>[2x]MLANENSLLTMFRELGSGKLPLQIEQFERGKTIFFPGDPAERVYLLVKGAVKLSRVYESGEEITVALLRENSVFGVLSLLTGQRSDRFYHAVAFT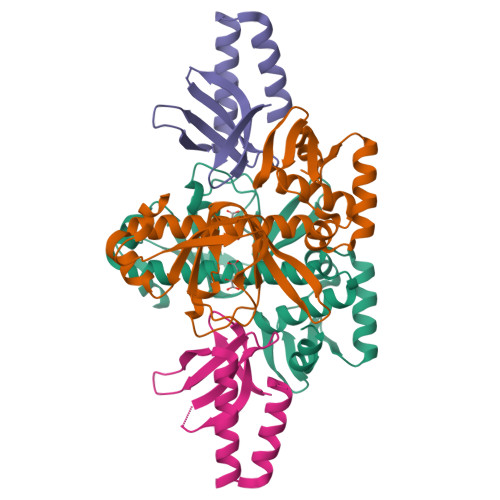PVQLFSVPIEFMQKALIERPELANVMLQGLSSRILQTEMMIETLAHRDMGSRLVSFLLILCRDFGIPSPDGITIDLKLSHQAIAEAIGSTRVTVTRLLGDLRESKLIAIHKKRITVFNPVALSQQFS;>MASENYLNHPTFGLLYQICSFGDSKELFATLYAQRLFFLVAFDARGTRFEPIGRNEARMLVDNRLRQLRRDASLQEYNQLQQVFKQTFL[2x]>MSDSKEVPSLPFLRHLLEELDSHEDSLLLFLCHDAAPGCTTVTQALCSLSQQRKLTLAALVEMLYVLQRMDLLKSRFGLSKEGAEQLLGTSFLTRYRKLMVCVGEELDSSELRALRLFACNLNPSLSTALSESSRFVELVLALENVGLVSPSSVSVLADMLRTLRRLDLCQQLVEYEQQEQARYRYCYAASP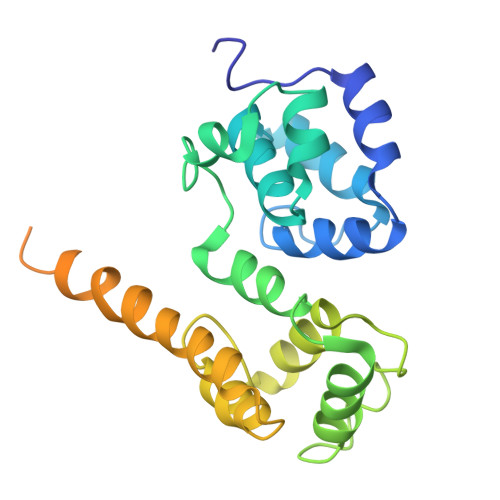SLPVRTLRRGHGASEHEQLCMPVQESSDSPELLRTPVQESSSDSPEQTTLEHHHHHH[4x]~{N}-[[(2~{R},3~{S},4~{R},5~{R})-5-[2-azanyl-6-oxidanylidene-7-(phenylmethyl)-1~{H}-purin-7-ium-9-yl]-3,4-bis(oxidanyl)oxolan-2-yl]methyl]-1,1,1-tris(fluoranyl)methanesulfonamide | 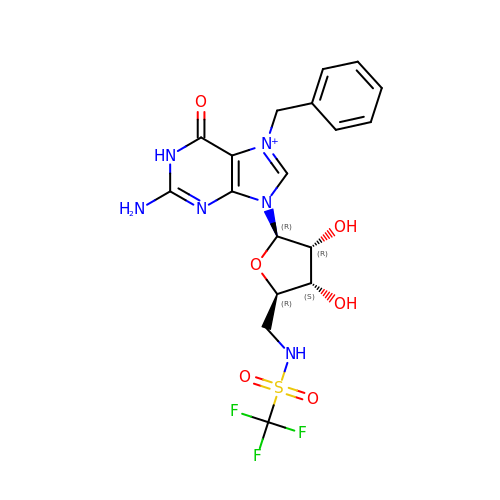C18 H20 F3 N6 O6 S | NMFHLBUCTTXCHX-XNIJJKJLSA-O>MATKKATMIIEKDFKIAEIDKRIYGSFIEHLGRAVYGGIYEPGHPQADENGFRQDVIELVKELQVPIIRYPGGNFVSGYNWEDGVGPKEQRPRRLDLAWKSVETNEIGLNEFMDWAKMVGAEVNMAVNLGTRGIDAARNLVEYCNHPSGSYYSDLRIAHGYKEPHKIKTWCLGNAMDGPWQIGHKTAVEYGRIACEAAKVMKWVDPTIELVVCGSSNRNMPTFAEWEATVLDHTYDHVDYISLHQYYGNRDNDTANYLALSLEMDDFIRSVVAIADYVKAKKRSKKTIHLSFDEWNVWYHSNEADKLIEPWTVAPPLLEDIYNFEDALLVGCMLITLMKHADRVKIACLAQLVNVIAPIMTEKNGPAWKQTIYYPFMHASVYGRGVALHPVISSPKYDSKDFTDVPYLESIAVYNEEKEEVTIFAVNRDMEDALLLECDVRSFEDYRVIEHIVLEHDNVKQ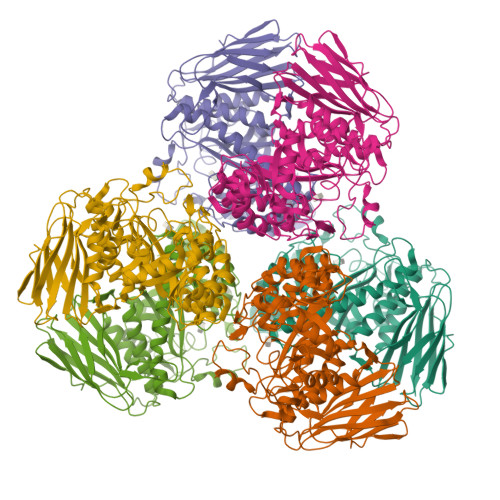TNSAQSSPVVPHRNGDAQLSDRKVSATLPKLSWNVIRLGKR[2x]>[2x]IIGGRESRPHSRPYMAYLQIQSPAGQSRCGGFLVREDFVLTAAHCWGSNINVTLGAHNIQRRENTQQHITARRAIRHPQYNQRTIQNDIMLLQLSRRVRRNRNVNPVALPRAQEGLRPG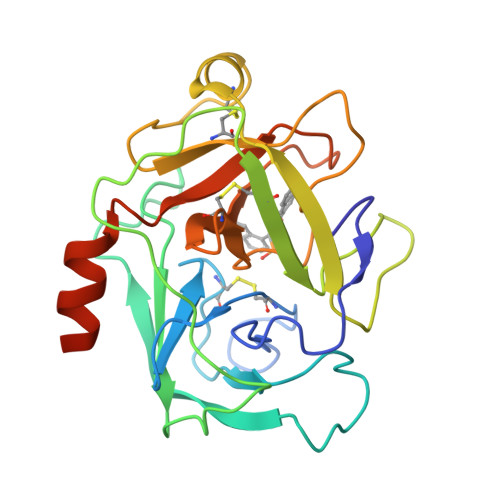TLCTVAGWGRVSMRRGTDTLREVQLRVQRDRQCLRIFGSYDPRRQICVGDRRERKAAFKGDSGGPLLCNNVAHGIVSYGKSSGVPPEVFTRVSSFLPWIRTTMRSFKLLDQMETPL> GSRESTGYLEELEKERSLLLADLDKEEKEKD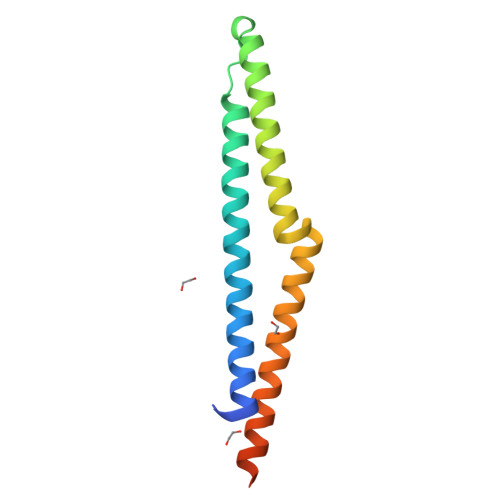WYYAQLQNLTKRIDSLPLTENFSLQTDMTRRQLEYEARQIRVAMEEQLGTCQDMEKRAQRRIARIQQIEKDILRIRQLLQSQATEAERSSQNKH> GHMNANLPPSAISELHGPRLLLRAWRDSDREAFAEMCADPQVMEFFPSVLDRAQS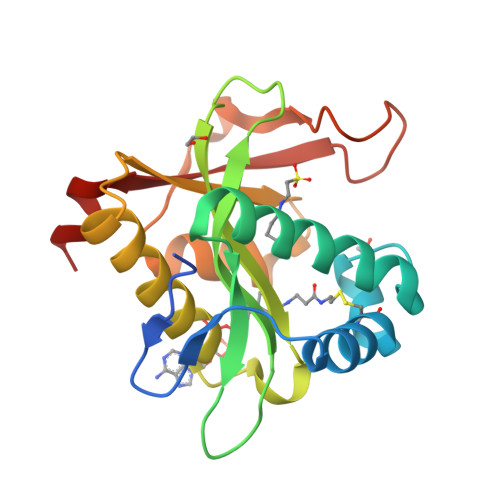DALVDRVQAHFAERGYGPWALELPGEAAFIGFTGLFDVTMDVHFAPTVEIGWRLAPAYWGRGLAREAAETALDFAFERLRLPEVVAFTTPPNRRSWGLMERLGMRRDPAEDFDHPLLAADHPMRRHILYRVDAARWAER> AFNNNPSSVGAYSSGTYRNLAQEMGKTNIQQKVNSTFDNMFGYNNTQQLYYPYTENGVYKAHYIKAINPDEGDDIRTEGQSWGMTAAVMLNKQEEFDNLWRFAKAYQKNPDNHPDAKKQGVYAWKLKLNQNGFVYKVDEGPAPDGEEYFAFALLNASARWGNSGEFNYYNDAITMLNTIKNKLMENQIIRFSPYIDNLTDPSYHIPAFYDYFANNVTNQADKNYWRQVATKSRTLLKNHFTKVSGSPHWNLPTFLSRLDGSPVIGYIFNGQANPGQWYEFNAWRVIMNVGLDAHLMGAQAWHKSAVNKALGFLSYAKTNNSKNCYEQV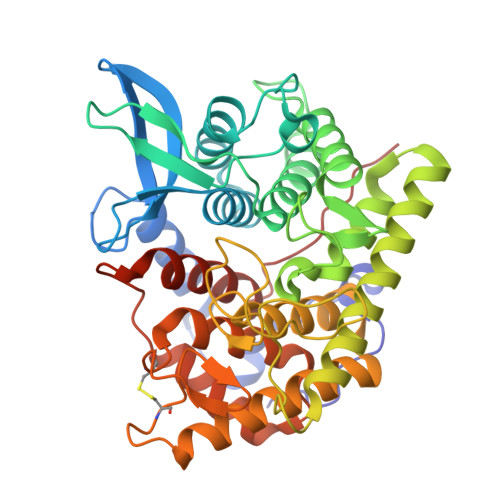YSYGGAQNRGCAGEGQKAANAVALLASTNAGQANEFFNEFWSLSQPTGDYRYYNGSLYMLAMLHVSGNFKFYNNTFN> MHADTA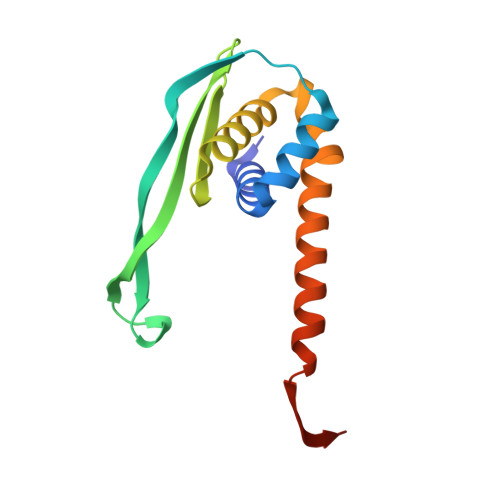TRQHWMSVLAHSQPAELAARLNALNITADYEVIRAAETGLVQIQARMGGTGERFFAGDATLTRAAVRLTDGTLGYSWVQGRDKQHAERCALIDALMQQSRHFQNLSETLIAPLDADRMARIAARQAEVNASRVDFFTMVRGDNA>MQERRALRLGVNGLPNSLEPVNAISNVGPRIVNQIFDTLIARDFFAKGAPGNAIDLVPALAESWERIDEKSVRFKLRQKVMFHDGVELTADDVAYTFSSERLWGPEAIKKIPLGKSYSLDFDEPVVEDKYTVTLRTKTPSYLIETFVASWMSRIVPKEYYKKLGAVDFGNKPVGTGPYKFVEFVAGDRVVLEANDAYWGPKPTASKITYQIVAEPATRVAGLISGEYDIITTLTPDDIQLINSYPDLETRGTLIENFHMFTFNMNQEVFKDKKLRRALALAVNRPIMVEALWKKQASIPAGFNFPNYGETFDPKRKAMEYNVEEAKRLVKESGYDGTPITYHTMGNYYANAMPALMMMIEMWKQIGVNVVMKTYAPGSFPPDNQTWMRNWSNGQWMTDAYATIVPEFGPNGQVQKRWGWKAPAEFNELCQKVTVL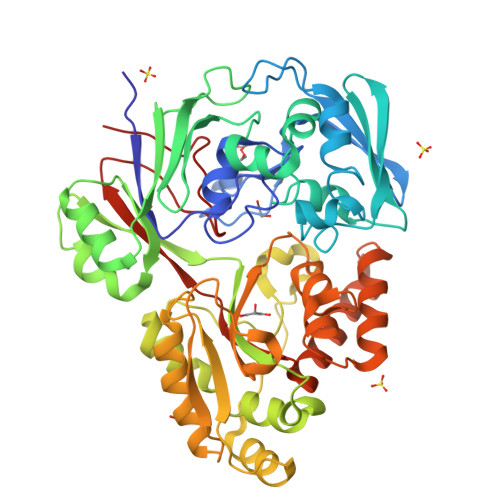PNGKERFDAYNRMRDIFEEEAPAVILYQPYDVYAARKDVHWKPVSFEMMEFRNNLSFGHHHHHH[4x]>[4x]MNTPEHMTAVVQRYVAALNAGD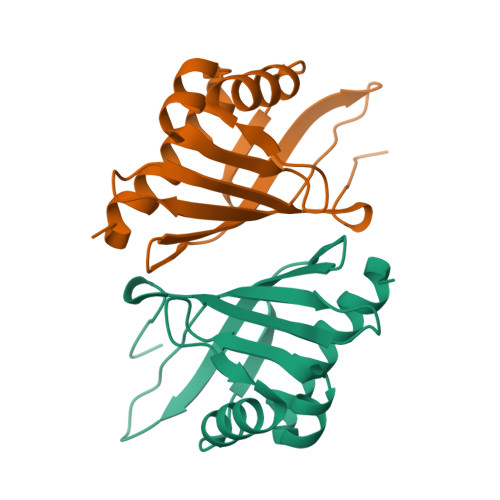LDGIVALFADDATVEDPVGSEPRSGTAAIREFYANSLKLPLAVELTQEVRAVANEAAFAFIVSFEYQGRKTVVAPIDHFRFNGAGKVVSMRALWGEKNIHAGA> PSGFNVVIEHDSEYQPDVKVTYYKNSIGTEANGFDTGPVFGG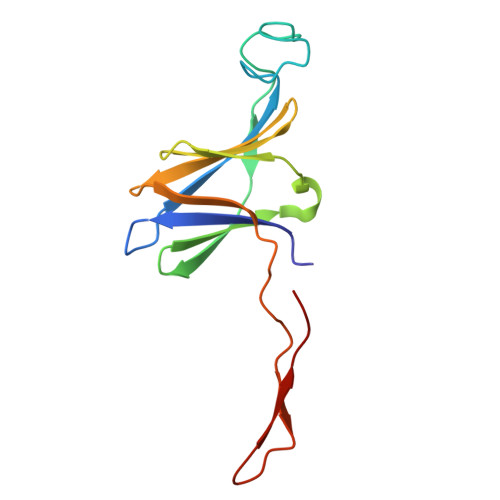ERIYNLASSLSYIRNKINVELPSVYAMAGEVVNNGNELLLINGTEIMRFVIEGATITKGYVEKVKPPTNLIVSDVTSTSAKISWENGG> AALGVQSINWQTAFNRQAHHTDKFSSQELILRRGQNFQVLMI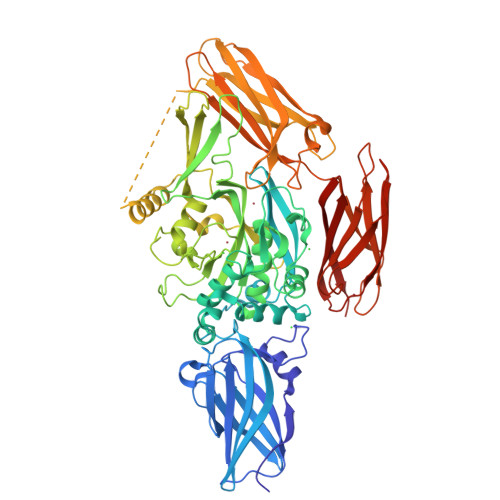MNKGLGSNERLEFIVSTGPYPSESAMTKAVFPLSNGSSGGWSAVLQASNGNTLTISISSPASAPIGRYTMALQIFSQGGISSVKLGTFILLFNPWLNVDSVFMGNHAEREEYVQEDAGIIFVGSTNRIGMIGWNFGQFEEDILSICLSILDRSLNFRRDAATDVASRNDPKYVGRVLSAMINSNDDNGVLAGNWSGTYTGGRDPRSWDGSVEILKNWKKSGLSPVRYGQCWVFAGTLNTALRSLGIPSRVITNFNSAHDTDRNLSVDVYYDPMGNPLDKGSDSVWNFHVWNEGWFVRSDLGPSYGGWQVLDATPQERSQGVFQCGPASVIGVREGDVQLNFDMPFIFAEVNADRITWLYDNTTGKQWKNSVNSHTIGRYISTKAVGSNARMDVTDKYKYPEGSDQERQVFQKALGKLKPNTPFAATSSMGLETEEQEPSIIGKLKVAGMLAVGKEVNLVLLLKNLSRDTKTVTVNMTAWTIIYNGTLVHEVWKDSATMSLDPEEEAEHPIKISYAQYERYLKSDNMIRITAVCKVPDESEVVVERDIILDNPTLTLEVLNEARVRKPVNVQMLFSNPLDEPVRDCVLMVEGSGLLLGNLKIDVPTLGPKERSRVRFDILPSRSGTKQLLADFSCNKFPAIKAMLSIDVAE>GVPGALSNQPAPPNEAPIATP[5x];>MALLNIFDIAGSALAAQSKRLNVAASNLANADSVTGPDGQPYRAKQVVFQVDAAPGQATGGVKVASVIESQAPEKLVYEPGNPLADANGYVKMPNVDVVGEMVNTMSASRSYQANIEVLNTVKSMMLKTLTLGQ[6x];>[5x]MLDRLDAALRFQQEALNLRAQRQE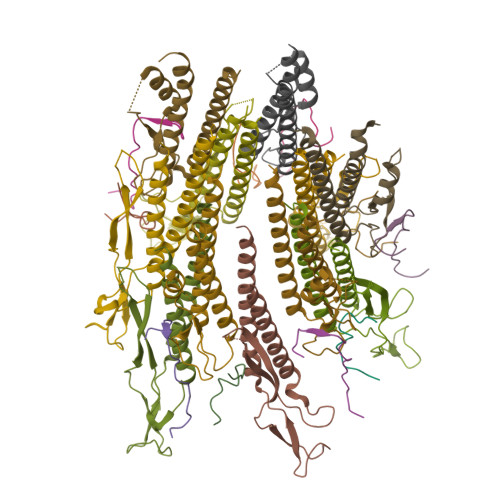ILAANIANADTPGYQARDIDFASELKKVMVRGREETGGVALTLTSSHHIPAQAVSSPAVDLLYRVPDQPSLDGNTVDMDRERTQFADNSLKYQMGLTVLGSQLKGMMNVLQGGN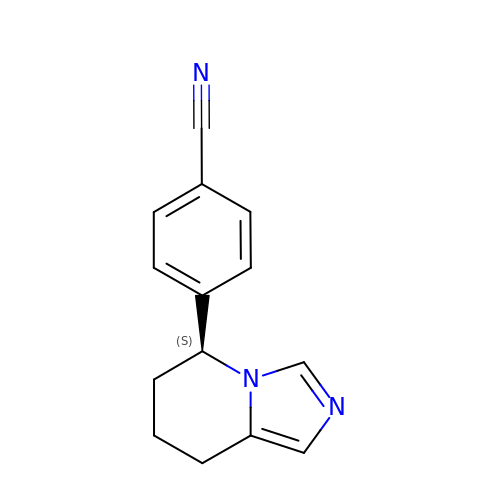4-[(5S)-5,6,7,8-tetrahydroimidazo[1,5-a]pyridin-5-yl]benzonitrile | C14 H13 N3 | CLPFFLWZZBQMAO-AWEZNQCLSA-N N-cycloheptylglycyl-N-(4-carbamimidoylbenzyl)-L-prolinamide 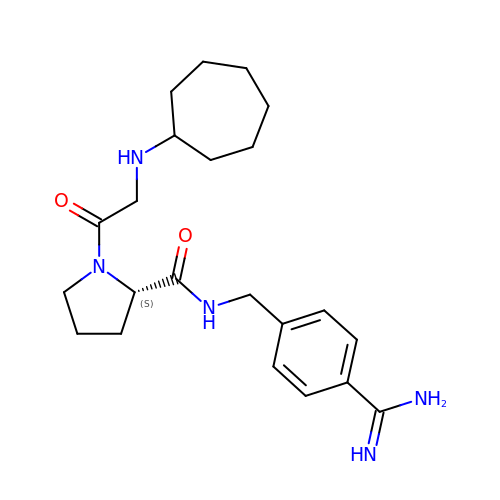| C22 H33 N5 O2 | BYTJPDBCLWUEBU-IBGZPJMESA-N The ferrous iron and 2-oxoglutarate (2OG)-dependent HIF prolyl hydroxylases (PHDs/EGLNs) catalyse trans-4-prolyl hydroxylations on HIFα subunits, thus promoting their binding to the von Hippel–Lindau protein (VHL), a targeting component of a ubiquitin E3 ligase, and signalling for HIFα degradation under normoxic conditions. The PHD-catalysed hydroxylations of HIF-1α/HIF-2α in higher animals occur in amino- and carboxy-terminal oxygen-dependent degradation domains (NODD and CODD). The three human PHDs exhibit different NODD/CODD selectivities, with PHD3 being substantially more selective for CODD than PHD1/2 (refs 16). Biophysical analyses employing crystallography and NMR reveal that the molecular basis of PHD isoform and variant selectivity involves enzyme–substrate interactions involving β2/β3 loop residues (that bind the LXXLAP motif) and helices α3 and α4, regions which display sequence variations between the PHD isoforms.

Comparison of the ODD complex structures and those without substrate reveals clear differences in NODD/CODD binding, especially in β2/β3 loop and C-terminal regions.

> GSHMASPNGQTKPLPALKLALEYIVPAMNKHGICVVDDFLGKETGQQIGDEVRALHDTGKFTDGQLVSQKSDSSKDIRGDKITWIEGKEPGCETIGLLMSSMDDLIRHCNGKLGSYKINGRTKAMVACYPGNGTGYVRHVDNPNGDGRCVTCIYYLNKDWDAKVSGGILRIFPEGKAQFADIEPKFDRLLFFWSDRRNPHEVQPAYATRYAITVWYFDADERAAAKVKYLTGEKGVRVELNKPSDSVGKDVF> MVLGKVKSLTISFDCLNDSNVPVYSSGDTVSGRVNLEVTGEIRVKSLKIHARGHAKVRWTESRNAGSNTAYTQNYTEEVEYFNHKDILIGHERDDDNSEEGFHTIHSGRHEYAFSFELPQTPLATSFEGRHGSVRYWVKAELHRPWLLPVKLKKEFTVFEHIDINLEHH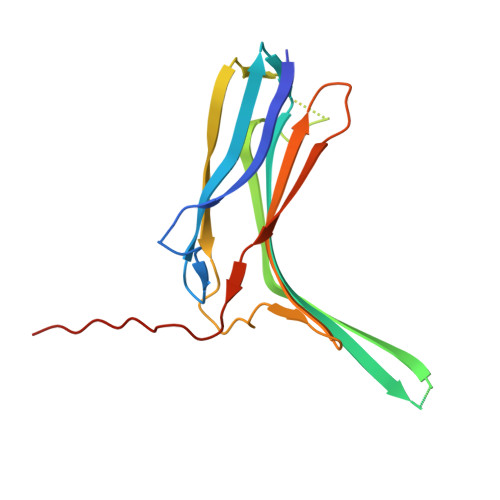HHHH2-KETO-DEOXY-GALACTOSE 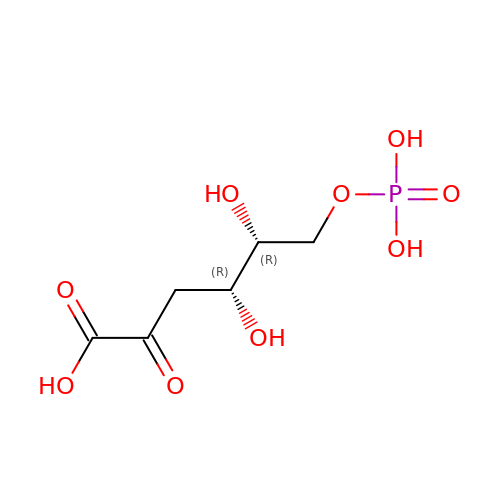| C6 H11 O9 P | OVPRPPOVAXRCED-NQXXGFSBSA-N>[2x]MQDVRVQVLPEVRGQLGGTVELPCHLLPPVPGLYISLVTWQRPDAPANHQNVAAFHPKM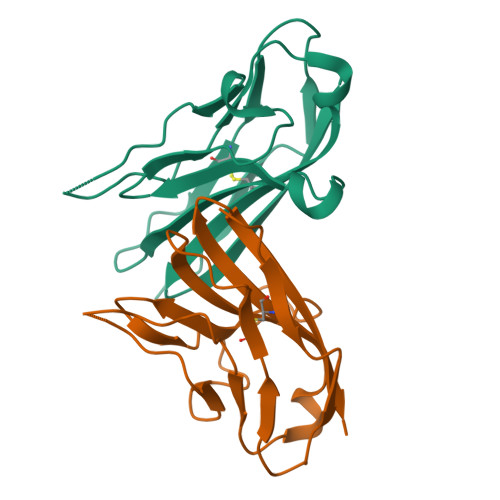GPSFPSPKPGSERLSFVSAKQSTGQDTEAELQDATLALHGLTVEDEGNYTCEFATFPKGSVRGMTWLRV>[6x]MPPHGELQYLGQIQHILRCGVRKDDRTGTGTLSVFGMQARYSLRDEFPLLTTKRVFWKGVLEELLWFIKGSTNAKELSSKGVKIWDANGSRDFLDSLGFSTREEGDLGPVYGF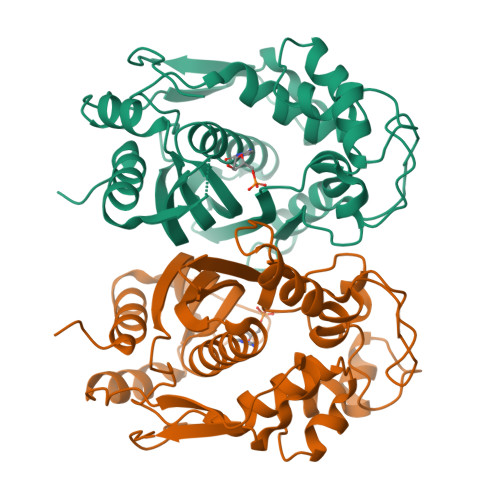QWRHFGAEYRDMESDYSGQGVDQLQRVIDTIKTNPDDRRIIMCAWNPRDLPLMALPPCHALCQFYVVNSELSCQLYQRSGDMGLGVPFNIASYALLTYMIAHITGLKPGDFIHTLGDAHIYLNHIEPLKIQLQREPRPFPKLRILRKVEKIDDFKAEDFQIEGYNPHPTIKMEMAV>PYPFKLPDLGYPYEALEPHIDAKTMEIHHQKHHGAYVTNLNAALEKYPYLHGVEVEVLLRHLAALPQDIQTAV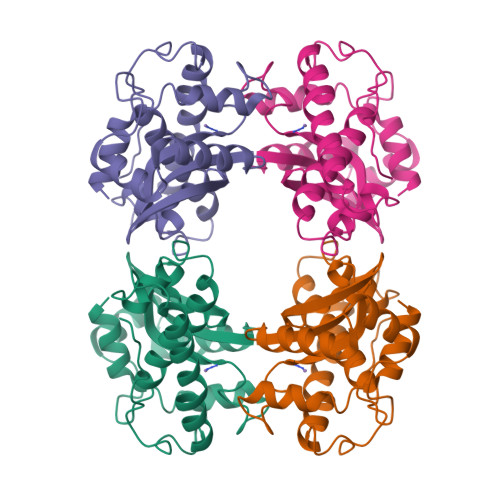RNNGGGHLNHSLFWRLLTPGGAKEPVGELKKAIDEQFGGFQALKEKLTQAAMGRFGSGWAWLVKDPFGKLHVLSTPNQDNPVMEGFTPIVGIDVWEHAYYLKYQNRRADYLQAIWNVLNWDVAEEFFKKA[2x]>[10x]MNIIAILNHMGVYFKEEPIRELHKALEALDFQIVYPNDREDLLKLIDNNARLCGVIFDWDTYNLDLCEEISAMNEHLPVYAFANTHSTLDVSLNDLRLNVEFFEYALGAAQDIAQKIRQSTDAYIDEILPPLTKALFNYVKEGKYTFCTPGHMGGTAFQKSPVGSIFYDFFGANAMKSDISISVGELGSLLDHSGPHKEAEEYIARTFNAERSYMVTNGTSTANKIVGMYSAPAGSTVLIDRNCHKSLTHLM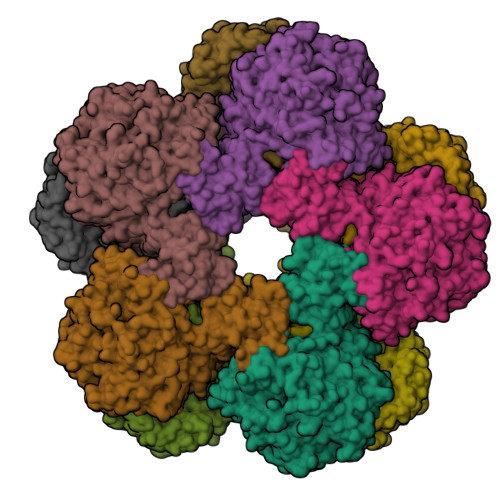MMSDITPIYFRPTRNAYGILGGIPKSEFQHDTIAERVAQTPNATWPVHAVVTNSTYDGLLYNTDYIKEALDVKSIHFDSAWVPYTNFSPIYKGLCGMSGGRVEGKVIYETQSTHKLLAAFSQASMIHVKGDINEETFNEAYMMHTSTSPHYGIVASTETAAAMMKGNAGKRLINGSIERAIRFRKEIKRLNSESEGWFFDVWQPEGIDEAKCWPLDSKDNWHGFKDIDNDHMYLDPIKVTLLTPGMQKDGSMADTGIPASIVSKYLDEHGIIVEKTGPYNMLFLFSIGIDKTKALSLLRALTDFKRSYDLNLRVKNMLPSLYREDPEFYENMRIQELAQGIHALIQHHNLPDLMYRAFEVLPTMVMNPHAAFQMELRGQTEEVYLEEMIGKVNANMILPYPPGVPLVMPGEMLTEESRPVLEFLQMLCEIGAHYPGFETDIHGAYRQADGRYTVKVIK> GSSMKASSGDQGSPPCFLRRPRPVRVVSGAEAE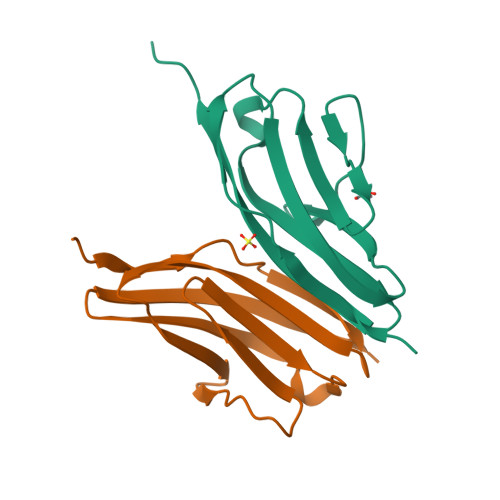LKCVVLGEPPPVVVWEKGGQQLAASERLSFPADGAEHGLLLTAALPTDAGVYVCRARNAAGEAYAAAAVTVLEPPA;> GSSRGIPPKIEALPSDISIDEGKVLTVACAFTGEPTPEVTWSCGGRKIHSQEQGRFHIENTDDLTTLIIMDVQKQDGGLYTLSLGNEFGSDSATVNIHIRSI>[2x]KIPKDTLIIAVENEIARINPAYSEDHDAVINLVFSGLTRFDENMSLKPDLAKSWDISKDGLVYDIFLRDDVLWHDGVKFSADDVKFSIEAFKNPKNNSSIYVNFEDIKSVEILNPSHVKITLFKPYPAFLDALSI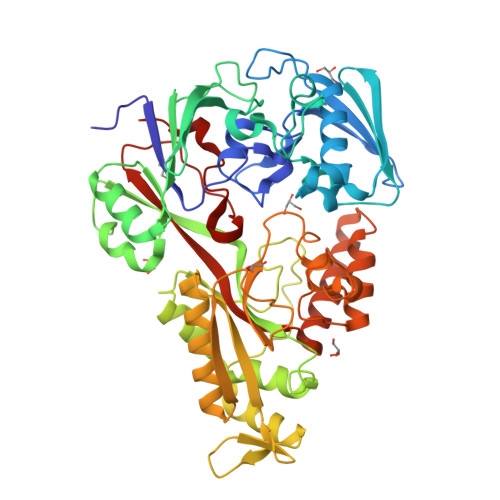GMLPKHLLENENLNTSSFNQNPIGTGPYKFVKWKKGEYVEFKANEHFYLDKVKTPRLIIKHIFDPSIASAELKNGKIDAALIDVSLLNIFKNDENFGILREKSADYRALMFNLDNEFLKDLKVRQALNYAVDKESIVKNLLHDYAFVANHPLERSWANSKNFKIYKYDPKKAEDLLVSAGFKKNKDGNFEKDGKILEFEIWAMSNDPLRVSLAGILQSEFRKIGVVSKVVAKPAGSFDYSKVDSFLIGWGSPLDPDFHTFRVFESSQDSALNDEGWNFGHYHDKKVDIALQKARNTSNLEERKKYYKDFIDALYENPPFIFLAYLDFALVYNKDLKGIKTRTLGHHGVGFTWNVYEWSK>MEKKKKLILFDFDSTLVNNETIDEIAREAGVEEEVKKITKEAMEGKLNFEQSLRKRVSLLKDLPIEKVEKAIKRITPTEGAEETIKELKNRGYVVAVVSGGFDIAVNKIKEKLGLDYAFANRLIVKDGKLTGDVEGEVLKENAKGEILEKIAKIEGINLEDTVAVGDGANDISMFKKAGLKIAFCAKPILKEKADICIEKRDL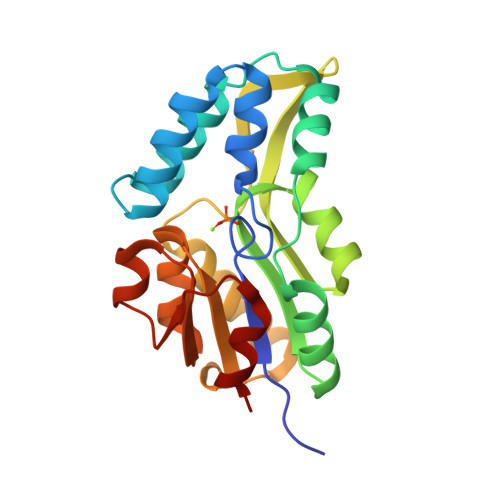REILKYIK[2x]> MIAEELLRAGRLDDALKALQEQVRSQPSNATLRIFLFQLLAVMGQWARAQNQLKVVGELDASALPMVQTYSTAIDCEALRREVFAGRLTPVILGQPAEWIAPLLQALSLDAEGHGEAAQALREQAFDAAPAVPGRIGEAPFAWLADADTRLGPVLEVIVNGRYAWLPMSNLRSLKVEAPSDLRDLVWLPAELTLANGGATVALLPARYAETVEHGDDAARLGRKTEWLDSGLPVGQRLFVTDAGETALFDLRELDFEPTDA;> MGSTTSSQKFIARNRAPRVQIEYDVELYGAEKKVQLPFVMGVMADLAGKPAEPQAAVADRKFLEIDVDNFDARLKAMKPRVAFNVPNVLTGEGNLSLDITFESMDDFSPAAVARKVDSLNKLLEARTQLANLLTYMDGKTGAEEMIMKAIKDPALLQALASAPKPKDDEPQA

The type VI secretion system (T6SS) is a bacterial nanomachine for the transport of effector molecules into prokaryotic and eukaryotic cells. It involves the assembly of a tubular structure composed of TssB and TssC that is similar to the tail sheath of bacteriophages. The AAA+ ATPase ClpV disassembles the contracted sheath, which resets the systems for reassembly of an extended sheath that is ready to fire again. The interaction of TagJ/HsiE with the sheath as well as with ClpV suggests an alternative mode of disassembly in which HsiE recruits the ATPase to the sheath.

We crystallized HsiE1 in complex with a peptide corresponding to the first 20 residues of HsiB1 (1MGSTTSSQKFIARNRAPRVQ20) or an HsiB1 degradation product, which appeared during purification of the E1-B1 complex. Both the E1-B1 peptide and E1-B1 fragment structures were solved by molecular replacement. In the E1-B1 complex structures, there is clear electron density for residues 8–20 of the extraneously added B1 peptide and for residues 8–30 of the co-purified B1 fragment, respectively. Both structures are nearly identical to the structure of HsiE1 alone, with an r.m.s. deviation of 0.4 Å in either case, and to each other with an r.m.s. deviation of 0.3 Å. The B1 fragment (residues 8–30) wraps around E1 in an extended conformation (main panel), following a prominent surface groove that originates in a deep hydrophobic pocket between the 12-stranded β-barrel of the “ImpE fold” and the two α-helices just preceding it (left inset). The B1 residue Phe10 nestles in that pocket, which is lined with residues Phe154, Trp171, and Pro181. The amino group of Lys9 of HsiB1 interacts with the negative dipole of helix α7 and forms hydrogen bonds with two carbonyl oxygens at the end of that helix (residues 155 and 157). Another key residue for the interaction is Arg18 of B1, which forms two salt bridges with the carboxyl group of Glu273 in HsiE1 (top right inset). In addition, most of the E1-B1 binding interface is hydrophobic in nature, involving Ala12, Gln20, Tyr23, Val25, and Leu27 from B1. Here, we have solved the structure of HsiE1 in complex with residues 8–30 of the P. aeruginosa HsiB1.8-(4-azanylbutyl)-6-(2-chlorophenyl)-2-(methylamino)pyrido[2,3-d]pyrimidin-7-one | C18 H20 Cl N5 O | 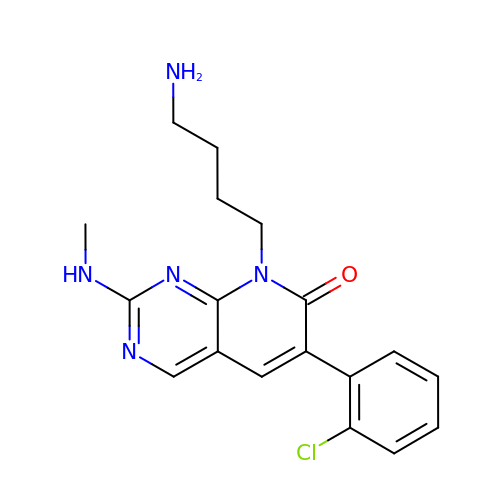DVQJNPZTPKFTFL-UHFFFAOYSA-N>MAITASPIQTFEQMKDNPIGLEMNVTTAVCEGFNIVLASFQALYLQYQKHHFVVEGSEFYQLHEFFSESYDEVQGHVHEIGERLNGLGGVPVASFSKLAELCCFTPEPDGVFSCRAMVEHDLSAEQEIIKVIRRQAGQAESLGDRAT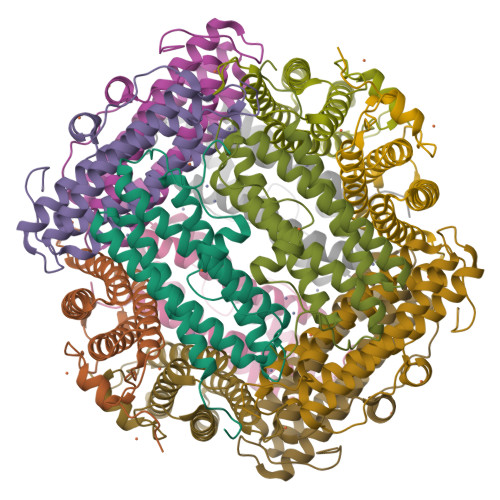RHLYEKILLESEDRAFHLSHFLAHDSLTPAFTLASQN[6x]> KRKSRWDETPASQMGG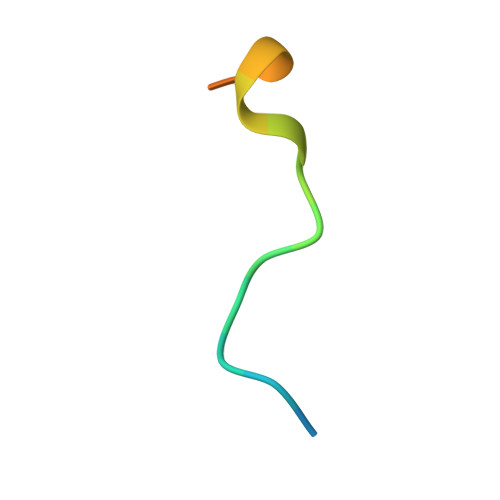STP> TRFTEEYQLFEELGKGAFSVVR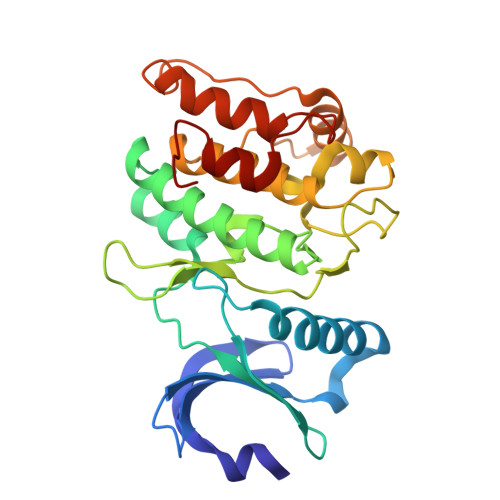RCVKVLAGQEYAAKIINTKKLSARDHQKLEREARICRLLKHPNIVRLHDSISEEGHHYLIFDLVTGGELFEDIVAREYYSEADASHCIQQILEAVLHCHQMGVVHRDLKPENLLLASKLKGAAVKLADFGLAIEVEGEQQAWFGFAGTPGYLSPEVLRKDPYGKPVDLWACGVILYILLVGYPPFWDEDQHRLYKQIKAGAYDFPSPEWDTVTPEAKDLINKMLTINPSKRITAAEALKHPWISHR The cannabinoid-1 and -2 receptors (CB1R and CB2R), both members of the lipid family of G protein coupled receptors (GPCRs), are the primary mediators of cannabinoid activity. Based on these expression profiles, and supported by animal studies, CB1R is thought to be the major target involved in the psychotropic and tetrad effects of cannabinoids, as well as their analgesic effects in tests of nociception, though because of the high similarity of the two receptors, and the peripheral distribution of CB2R, a role for the latter receptor often cannot be discounted without direct testing. The CB1R orthosteric site is large and lipophilic, explaining the high molecular weight and hydrophobicity of many of its ligands. In this work, we computationally dock a library of 74 million virtual but readily accessible molecules against human CB1R, revealing a range of different scaffolds with relatively favorable physical properties.

To understand the SAR of ‘1350 at atomic resolution, and to template future optimization, we determined the cryo-EM structure of the ‘1350-CB1R-Gi1 complex to a nominal resolution of 3.3 Å. Consistent with earlier structures of human CB1R in its activated state, the ligand occupies the orthosteric pocket formed by transmembrane helices (TMs) 2–3 and 5–7 and is capped by ECL 2. The experimental structure of ‘1350 superposes well on the docking-predicted pose of the R-enantiomer, which was the enantiomer with the better docking score to the receptor (-43 DOCK3.7 score versus -38 DOCK3.7 score for the S-enantiomer). In optical rotation studies, ‘1350 was shown to be the (-) enantiomer, together identifying ‘1350 as the R/(-) enantiomer. The predicted and experimental structures superposed with an all-atom RMSD of 0.78 Å. Despite the local resolution limit that prevents unambiguously modelling all rotamers, the density suggests that major interactions with CB1R predicted by the docking are likely preserved in the experimental structure, including the key hydrogen-bond between the amide carbonyl of the ligand and S3837.39. The trifluoromethyl group is complemented by van der Waals and quadrupole interactions with residues W2795.43 and T1973.33, as anticipated by the docked structure, and consistent with the improvement in affinity by -1.7 kcal/mol (‘51486 Ki = 731 nM vs. ‘60154 Ki = 44 nM, 17-fold increased Ki from CF3 addition only) on its replacement of the original fluorine. Key learnings from the SAR include the importance of bulky and hydrophobic groups in the R1 position, which is modeled to pack against W2795.43 and T1973.33, with a meta-substituted CF3 being most favorable. Further, methylation of the chiral center (R4 position, ‘1350, ‘4936, ‘5806) meaningfully improved affinity (approximately 6-fold in ‘4936, 15-fold in ‘5806, and 50-fold in ‘1350). This addition is predicted to increase van der Waals interactions between the ligands and transmembrane helix 2.

> DYKDDDDAMKSILDGLADTTFRTITTDLLYVGSNDIQYEDIKGDMASKLGYFPQKFPLTSFRGSPFQEKMTAGDNPQLVPADQVNITEFYNKSLSENLYFQGSFKENEENIQCGENFMDIECFMVLNPSQQLAIAVLSLTLGTFTVLENLLVLCVILHSRSLRCRPSYHFIGSLAVADLLGSVIFVYSFIDFHVFHRKDSRNVFLFKLGGVTASFTASVGSLFLTAIDRYISIHRPLAYKRIVTRPKAVVAFCLMWTIAIVIAVLPLLGWNCEKLQSVCSDIFPHIDETYLMFWIGVTSVLLLFIVYAYMYILWKAHSHAVRMIQRGTQKSIIIHTSEDGKVQVTRPDQARMDIRLAKTLVLILVVLIICWGPLLAIMVYDVFGKMNKLIKTVFAFCSMLCLLNSTVNPIIYALRSKDLRHAFRSMFPSCEGTAQPLDNSMGDSDCLHKHANNAASVHRAAESCIKSTVKIAKVTMSVSTDTSAEALGSHHHHHH>[2x]ASRYLTDMTLEEMSRDWFMLMPKQKVAGSLCIRMDQAIMDKNIILKANFSVIFDRLETLILLRAFTEEGAIVGEISPLPSLPGHTDEDVKNAV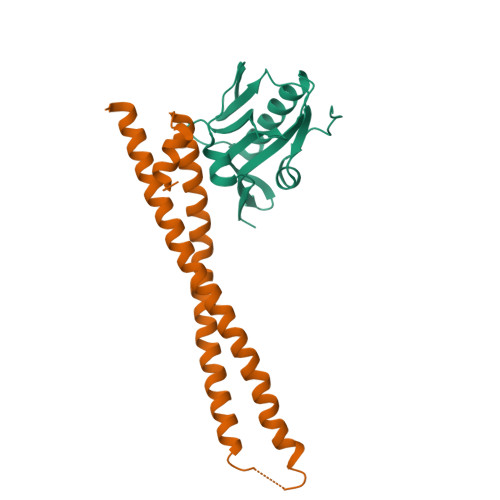GVLIGGLEANDNTVRVSETLQRFAWRSSNENGRPPLPPKQKRKMARTIKSEV;>GSKEDSVEAVGAQLKVYHQQYQDKSREYDQLYEEYTRTSQELQMKRTAIEAFNETIKIFEEQGQTQEKSSKEYLERFRREGNEKEMQRILLNSERLKSRIAEIHESRTKLEQQLRAQASDNREIDKRMNSLKPDLMQLRKIRDQYLVWLTQKGARQKKINEWLGI[2x]>SMQELFNNLMELCKDSQRKFFYSDDVSASGRTYRIFSYNYASYSDWLLPDALECRGIMFEMDGEKPVRIASRPMEKFFNLNENPFTMNIDLNDVDYILTKEDGSLVSTYLDGDEILFKSKGSIKSEQALMANGILMNINHHRLRDRLKELAEDGFTANFEFVAPTNRIVLAYQEMKIILLNVRENETGEYISYDDIYKDATLRPYLVERYEIDSPKWIEEAKNAENIEGYVAVMKDGSHFKIKSDWYVSLHSTKSSLDNPEKLFKTII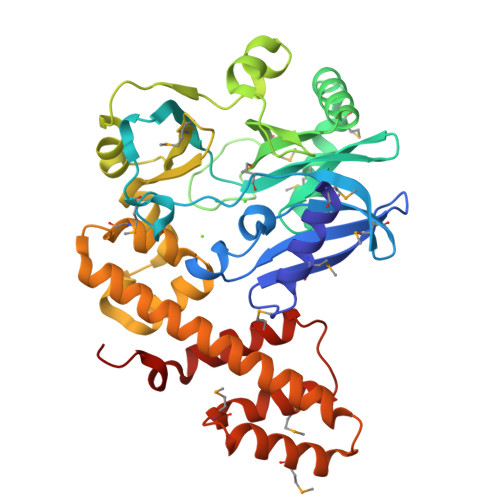DGASDDLKAMYADDEYSYRKIEAFETTYLKYLDRALFLVLDCHNKHCGKDRKTYAMEAQGVAKGAGMDHLFGIIMSLYQGYDSQEKVMCEIEQNFLKNYKKFIPEGY[2x]Human Eg5 (KSP, kinesin spindle protein, KIF11), a member of the kinesin-5 family, is a well characterized mitotic kinesin that is required to establish a bipolar mitotic spindle. Eg5 forms homotetramers that can attach to neighbouring antiparallel spindle MTs and slide them against each other, thus separating the duplicated centrosomes. Loss of Eg5 function owing to RNA interference or small-molecule inhibitors results in the formation of monoastral spindles, cell-cycle arrest and apoptosis. A number of small-molecule inhibitors of Eg5 have been identified, including MK-0731, pyrrolotriazin-4-one-based inhibitors and the quinazolin-4-­one-based ispinesib, all of which are allosteric inhibitors that bind to the unique L5 loop region of the catalytic domain.

Here, we report the 2.6 Å resolution structure of the ternary complex of the Eg5 motor domain in complex with Mg2+ADP and ispinesib. The data for the Eg5–ADP–ispinesib complex suffered from pseudo-mero­hedral twinning and revealed translational noncrystallographic symmetry, leading to challenges in data processing, space-group assignment and structure solution as well as in refinement. Depending on the molecule, the N-terminal 15–17 residues as well as the C-­terminal 2–9 residues of Eg51–368 are disordered, as are a number of loops; in particular, loops L10 and L11 are absent from all four molecules. All four molecules in the asymmetric unit depict the final ispinesib-bound state. Helix α4 rotates and moves by around 7 Å in the inhibitor-bound state compared with the native structure. The benzyl moiety of the ligand is buried deeply in the hydrophobic part of the pocket, where it stacks with the Pro137 ring and makes an edge-to-face interaction with the side chain of Trp127, as well as hydrophobic interactions with the side chains of Tyr211 and Leu214. In addition, the benzyl group also forms an intramolecular edge-to-face stacking interaction with the p-­toluyl moiety of the inhibitor, which in turn stacks extensively with the mostly flat protein backbone of Glu118/Arg119 and also interacts with parts of the side chains of Arg119, Trp127 and Asp130. The chlorine substituent of the 7-chloro-3,4-dihydro-4-oxo-3-­(phenylmethyl)-2-quinazolinyl moiety sits in another mostly hydrophobic pocket formed by the backbone of Gly217 and the side chains of Leu160, Leu171 and Arg221. In three of the four chains (B/C/D) the primary amine of ispinesib is oriented towards the ADP-binding site, and while it is mostly solvent-exposed the amine can interact favourably with the anionic Glu116 side chain.

>[4x]GPMASQPNSSAKKKEEKGKNIQVVVRCRPFNLAERKASAHSIVECDPVRKEVSVRTGGLADKSSRKTYTFDMVFGASTKQIDVYRSVVCPILDEVIMGYNCTIFAYGQTGTGKTFTMEGERSPNEEYTWEEDPLAGIIPRTLHQIFEKLTDNGTEFSVKVSLLEIYNEELFDLLNPSSDVSERLQMFDDPRNKRGVIIKGLEEITVHNKDEVYQILEKGAAKRTTAATLMNAYSSRSHSVFSVTIHMKETTIDGEELVKIGKLNLVDLAGSENIGRSGAVDKRAREAGNINQSLLTLGRVITALVERTPHVPYRESKLTRILQDSLGGRTRTSIIATISPASLNLEETLSTLEYAHRAKNILNKPEVNQK>[2x]GAMDPREVILCKDQDGKIGLRLKSIDNGIFVQLVQANSPASLVGLRFGDQVLQINGENCAGWSSDKAHKVL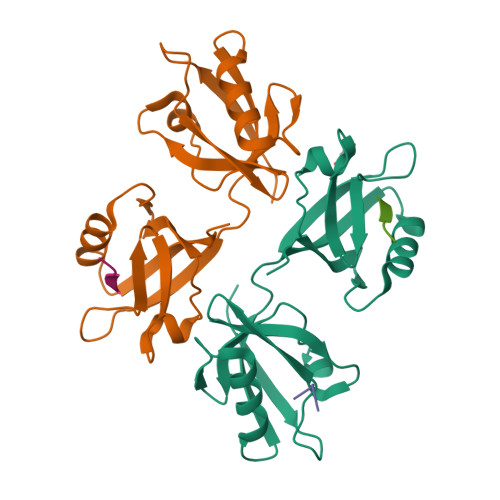KQAFGEKITMTIRDRPFERTITMHKDSTGHVGFIFKNGKITSIVKDSSAARNGLLTEHNICEINGQNVIGLKDSQIADILSTSGTVVTITIMPAF;>[3x]TNEFYF> SMANTIKVEGYPSMEWPTSLDIPLKASEELVGIDLETDLPDDPTDLKTLLVEESSEKEHWLTIALAYCNHGKTNEGIRLIEMALDVFQNSERASLHTFLTWAHLNLAKGHSLSVETKEHELTQAELNLKDAIGFDPTWIGNMLATVELYYQRGHYDKALETSDLFVKSI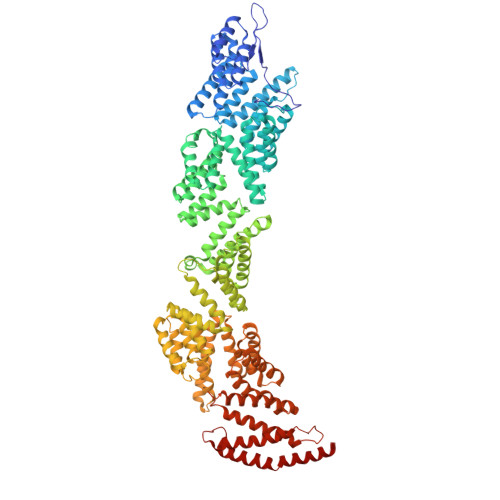HAEDHRSGRQSKPNCLFLLLRAKLLYQKKNYVASLKIFQELLVINPVLQPDPRIGIGLCFWQLKDPKMAIKSWQRALQINSKNTSASILVLLGEFHNSLTDSTNDEVFKETFSKALSDLKNIFSENQNNPVLLTLLQTYHYFKGDFQTVLDIYHHKILKMSPLIAKTVLSESSFWCGRAHYALGDYRKSFIMFQESLKKNEDNLMARLGLGQTQIKSNLLEESIITFENLYKTNESLQELNYILGLLYAGKTLDVKTSKSIPAKELNKLNEKALQYLERYIKLTVAKKNQLIISRVYLVISQLYESQNQYKISLDFLSKALEEMEFVNKDEVPLEILNNLACYHFINGDLTKADNLFEQAKAKVSDMNKSVNITLEYNIARTSEKTNWEKSESIYSQITSSHPSYISARIRNLYIKFAHSKINDSEMNIEINGLLEMNKSDLEMRSFYGWYLKNSEERKNSEKSTSHNKETLVKYNSHDAYALISLANLYVTIARDGKKSRNPKEQEKSKHSYLKAIQLYQKVLQIDPFNVFAAQGVAIIFAESKRLGPALEILRKIRDSLDNEDVQLNLAHCLLEMREFGKAIENYELVLKKFDNERTRPHILNLLGRAWYSRGMKERSVSFFQKALENAKTALELFVQQSAKNKFIHSVKFNIALLQFQIAETLRRSNPKFRTVQQIKDSLEGLEEGLALFKELNDLKEFNMIPKEELEQRIQLGETTMKSALERSLNEQEEFEKDQ>[2x]MKLAVAGKGGVGKTTVAAGLIKIMASDYDKIYAVDGDPDSCLGQTLGLSIEEAYAITPLIEMKDEIREKTGDGGLLILNPKVDGDLDKYGRYIDDKIF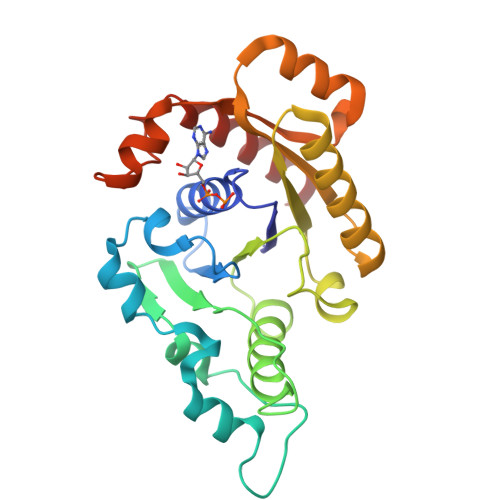LIRMGEIKKGGSQCYCRENSFLGSVVSALFLDKKEAVVMDMGAGIEHLTRGTAKAVDMMIAVIEPNLNSIKTGLNIEKLAGDLGIKKVRYVINKVRNIKEEKLIKKHLPEDKILGIIPYNELFIELSLKGEEIWQSTNPAFVNLHDIYQKLRLEVG> XG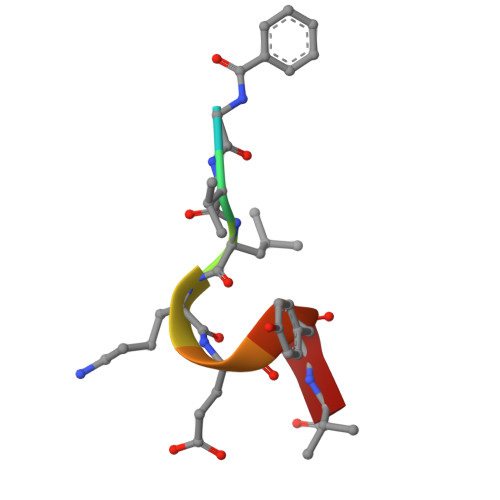VLKEYGV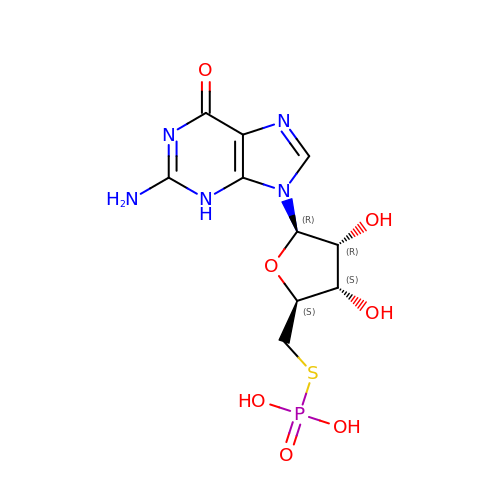5'-S-phosphono-5'-thioguanosine | C10 H14 N5 O7 P S | GPKODAQOVIGWBY-UUOKFMHZSA-N Among them one such target is β-clamp. β-clamp, a part of DNA pol III holoenzyme is very crucial protein as it is involved in myriads of steps during DNA replication. It is the key protein that increases the processivity of many important enzymes and complexes by interacting with them. β-clamp prevents the polymerase from dissociating, while polymerase’s rapid movement along the DNA molecule. Biological active form of β-clamp is dimer and each monomeric unit consists of three domains, where the protein-binding site resides in between domain II and III. This interaction site is divided into two subsites and all β-clamp interacting partners bind to these subsites.

All of these crystals yielded clear electron density for the ligand molecules with good occupancy, except for 5-chloroisatin. The occupancy of 5-chloroisatin was quite low. Moreover, based on data obtained from the soaked crystals, the temperature factor of this inhibitor was high when compared to the average temperature factor of the protein. Thr175 of Hpβ-clamp was also observed to make a hydrogen bond with the inhibitor 5-chloroisatin. In case of 5-chloroisatin, the Thr175 of Hpβ-clamp makes hydrogen bond with ligand however that in Ecβ-clamp is made by Thr172 in the neighborhood. Out of various hydrophobic contacts between the β-clamp and inhibitor, three of them are common in both H. pylori and E. coli β-clamp. These residues include Ile248, Lys176, Arg177 in Hpβ-clamp, and Val247, His175, Arg176 in Ecβ-clamp. The orientation of the 5-chloroisatin inhibitor in the docked structure did differ from that in the crystal structure, but this difference did not affect much the structure of the binding site. With an MIC of 18 µM drug C1 (5-chloroisatin) showed significant antimicrobial activity. The drug C1 (5-chloroisatin) showed extra H-bond with Thr173 compared to other complex structures may be responsible for better binding and thus better inhibition.

>[2x]MKISVSKNDLENALRYLQAFLDKKDASSIASHIHLEVIKEKLFLKASDSDIGLKSYIFTQSSDKEGVGTINGKKFLDIISCLKDSNIILETKDDSLAIKQNKSSFKLPMFDADEFPEFPVIDPKVSIEVNAPFLVDAFKKIAPVIEQTSHKRELAGILMQFDQKHQTLSVVGTDTKRLSYTQLEKISIHSTEEDISCILPKRALLEILKLFYENFSFKSDGMLAVIENEMHTFFTKLIDGNYPDYQKILPKEYISSFTLGKEEFKESIKLCSSLSSTIKLTLEKNNALFESLDSEHSETAKTSVEIEKGLDIEKAFHLGVNAKFFLEALNALGTTQFVLRCNEPSSPFLIQESLDEKQSHLNAKISTLMMPITL> GPLMSGLNDIFEAQKIEWHEGSAGGSGHMTDLRKLEALQALHAELVAVRQHRFEGLQVLETLLEEQTDAFKALIAKPARDTKDREALGKEPKKLKIGEEEYSLNEDFVNDCLKLADELDLNEKESARILIDCDAEGDVETQSRPLWECGVIRFHQERKYLLDCMRLILEIAADEDIDAGLQESFGVAAEDKIFGIPPPWERNKENQPTQVKKFIPRCMEAMKGVRSMLQCMADKANARNMLQ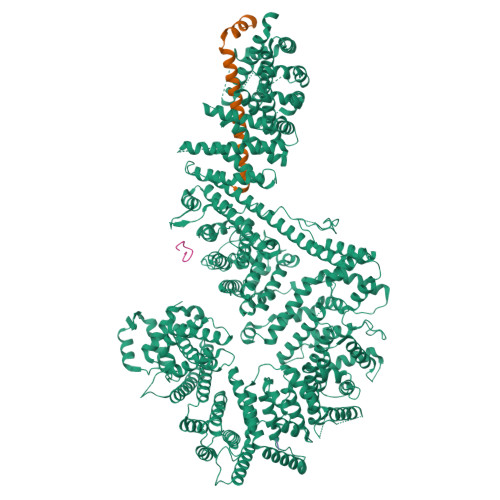QASLVRPLDNQETLDFSRLSLVEQHECLASILHAAVQRHHATIADFQDFIKILRKWDKYDHFLIHLIPVLAAYITEFGSPEGMGDLQQARRLNDFICKGGDEDSWALPVLGAAVRAWWIAEHNGFYLDDTVQDLRGINLDEEDEQRTKQFLDALKEGAFDFILSVAADCKAQEWQDPSQLGARQWLQRKIPSLPSEPFPFSHFLQHSLMVHLEGFVDATISNLPDVLRKLRTEEDEQRQLRPNHEQDMDLERFLIIISYAYEGRPDAAMSFWEDPDSNLAGFLQWASRRASTPLVSAFCEMLRCLADNEECATAAHNFLLDEGHQASGKMKRSQSLTWSQIFKELEYFTTKVCSERPNPPQASMHRPGRPGADPAEIEPESALMLECYLRLIAKLATESEIARKRLIMDEDFNLVDTILKLSVGVIPHRLRACIFYVLKALMIRKTHEELDAMWRWVEAWMTNPFSSLPGSQGAPQRISFLGQTPGPQECMEMMFREFGTGFEQSNAFIQLLTTLLVPPEGLNSLNDSVPFPEWLGSSIRTLGIEPYVDFVFDVFANRTKDISDPSQLRILRLSCLDFVMVCLVTFNEDLIVLGHESNISIDDAMAATNLATYVRLHPFSRVMEWLFNEKVITSLINTIHQDPISLGSASPDSPLVVSILRAIQVMIKALELQETYLHLVRPEVLRYQGEAGVRRKPVANAAYSAFEDGILSHLSLVVDLGKYCNLGHAELTLACLKLLEKISTSSRILSAWSPDSGRLGHRNKAIVQLERNGEGETISASLSASIMATLDPALAASGENYRVKLAILDFLYACLRATPDQPTIAHQLLGFHCELSKLGIEPKGPFDMQKSLFHSLLNVLITLTVSEEEQGMRGYLVTLKYRVLRILQLLWKSPLSASLVMDELRATNFLFHMLLREVQIQPQLPWDGQLVTGCEFLLSDASLAYIDYLASRAAIFEYIGKELCSVSQNRIPSIKRQIFDALNGQIFVDEEAPLTIPSIFDFFDFINTDYKWEEIPSPHFTYLKDLDLGPCILEHKYAGVHYDIRKAQEILALKRKEYEHSQLATPEFLETVELEEKVLIEWLTVRNRANLLLTARLNLLQAWANLLLVMIESNDFKSTPKMAFLLQALQAILPTLEAFSSLKSDEAFELARVAKVLLWKLDFSQDSDAGLDREQFTVGNLIGDKLFQLFQLCLSAISQCSGTPELRSLYYSICYRYLTAVVDNDATVAATPASSTIGPTRSVTNARARTLKAITLYGDRLLNVICDDAYGSDTTCQTAAMILLNALVHTSRASSAAGVSPADVDCPIIDALNRLNFIGVLVDSLKEILNEWLAPSSTFDPSLSTNASPSLPIPASPSQQYTSAKLALLLQLCQTRQGAKYVLQANLFRALEQSGVFAADPELVEVDSESGVPRVVALERHYALLVALARVVGAAVTARGAHNIVQGRKFLTQHRGLVVHVLKKNAGIGGGVVGNSLASSINGGSTATMTRRDEILAQQALEERIEELAEAFMLLITATGFLEYESEQVPSEQPRAHTTFFH;> SGTGLGEVDVDTYLSNLQTKTTLSMIADGLERSARDFDAFLEENVTLEWEAQRKRIYQHFGIK;> SATPLSGKAKVKSRSILPMYKLSPANASRLVTTPQKRAYGFSFSAYGSPTSPSSSASSTPGAFGQSILS;> SQQDGSLRSRKANLETGAFGKSTRRTRSKAATPAKRED>[2x]MQNIPPQVQAMLGQLDTYQQQLQLVIQQKQKVQADLNEAKKALEEIETLPDDAQIYKTVGTLIVKTTKEKAVQELKEKIETLEVRLNALNRQEQKINEKVKELTQKIQAALRPPTAG;> MIRMAQNNKELEKLAYEYQVLQAQAQILAQNLELL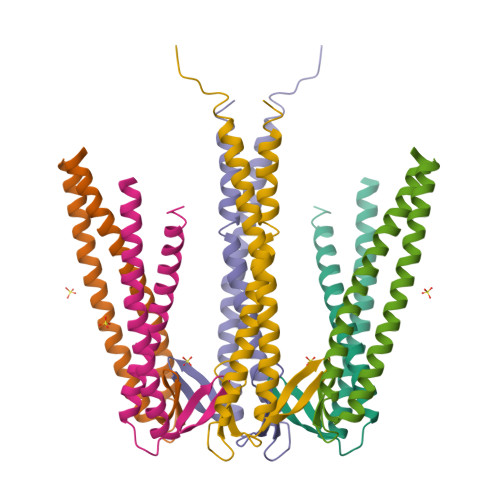NLAKAEVQTVRETLENLKKIEEEKPEILVPIGAGSFLKGVIVDKNNAIVSVGSGYAVERSIDEAISFLEKRLKEYDEAIKKTQGALAELEKRIGEVARKAQEVQQKQSMTSFKVKK>MSGSHHHHHHSGSMSERPSDLVVNRLVL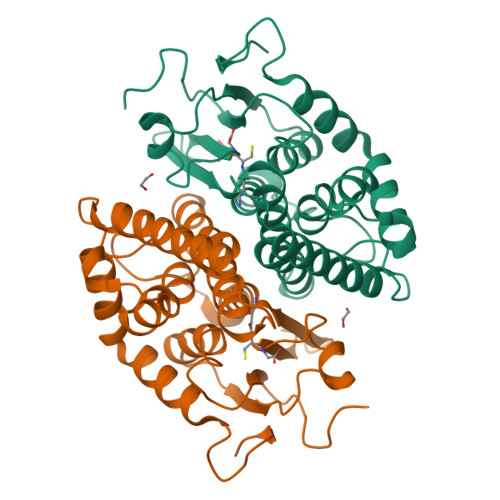FVVKGTATSTHNTVKPLILLEELGVPHDIYVVEKVSAPWFSEINPHKMVPAILDRSPDGRDTLRAWESTSTLMYIADAYDKDGTFGGRNVQERSEINNWLTLHTAALGPTAKYWLYFYKLHPEKLPKTIEKLRSNITVQYDILERRLNEPGQQYLALKDRPTIADIATLPFAMKSTAELFGLEFEKWPKLQEWSVRMGEREAVKRAWQRVAGFGHGEKEYGMLEA[6x]1, 4-Dihydroxy-2-naphthoyl-CoA (DHNA-CoA) synthase, also called MenB, is responsible for conversion of o-succinylbenzoyl-CoA to DHNA-CoA in the biosynthesis of both vitamin K1 and K2. It catalyzes a multiple-step intramolecular Claisen condensation reaction involving two high energy oxyanion intermediates and two keto-enol tautomerizations in the formation of a naphthenoid ring. The first crystal structure of DHNA-CoA synthase from Mycobacterium tuberculosis shows that it forms two eclipsed trimers organized in a homologous hexameric assembly, in which each monomer is comprised of an N-terminal spiral core domain and a C-terminal helical domain conforming to a canonical crotonase fold. In addition to observing the folding of the active-site loop into a well-defined structure as previously seen in the substrate analog complex structure, we have identified a significant reorientation of the C-terminal helix as an additional conformational change caused by the small molecule ligands.

Through symmetry operation, all the trimers are found to be a part of the hexameric quaternary structure of scMenB. The active site of scMenB in complex with HNA-CoA is closely similar to that of ecMenB in complex with HNA-CoA. The similarities include the hydrogen-bonding stabilization of the carbonyl oxygen in the ligand by backbone amides of Gly-77 and Gly-123, hydrophobic interactions between the aromatic ring in the ligand with side chains of Leu-96, Val-98, Leu-99, and the hydrogen bonding interaction between the phenolic hydroxyl of the ligand and the side-chain hydroxyl of Ser-151. In addition, there is also a hydrogen-bonding network interacting with C1-OH of HNA-CoA, which involves the carboxyl side chain of Asp-153, the backbone amide of Gly-123, three water molecules and the backbone carbonyl oxygen of Phe-152 (data not shown). Moreover, the hydroxyl groups of Tyr-87 from the ordered active-site loop and Tyr-248 from the opposing subunit also form a strong hydrogen bond with an O−H⋅⋅⋅O distance of 2.9 Å. Furthermore, in the scMenB: HNA-CoA structure a chloride ion occupies the bicarbonate binding site (data not shown), similar to that in the ecMenB:HNA-CoA complex. One of them is a strong hydrogen bond between the strictly conserved A-loop Arg-82 and the backbone carbonyl oxygen of the C-helix Gly-253, and the other polar loop-helix interaction is a hydrogen bond between the backbone carbonyl oxygen of Arg-82 and the side chain guanidinium group of Lys-257. In the scMenB complexes, the side chain benzene ring of Phe-260, which corresponds to ecMenB Phe-270, also forms hydrophobic contact with the adenine ring of the ligands. In addition, the adenylate 3′-phosphate group of the ligand is also stabilized by a ligand-induced salt bridge with the side chain of scMenB Lys-263, which is equivalent to ecMenB Lys-273.

>MDWHIAKHYDDILYYKAGGIAKIVINRPHKRNAFRPQTVFELYDAFCNAREDNRIGVVLLTGAGPHSDGKYAFCSGGDQSVRGEGGYIDDQGTPRLNVLDLQRLIRSMPKVVIALVAGYAIGGGHVLHLVCDLTIAADNAIFGQTGPKVGSFDGGFGSSYLARIVGQKKAREIWYLCRQYSAQEAERMGMVNTVVPVDRLEEEGIQWAKEILSKSPLAIRCLKAAFNADCDGQAGLQELAGNATLLYYMTEEGSEGKQAFLEKRPPDFSQYPWLP[9x]> ASLTEIEHLVQSVCKSYRETCQLRLEDLLRQRSNIFSREEVTGYQRKSMWEMWERCAHHLTEAIQYVVEFAKRLSGFMELCQNDQIVLLKAGAMEVVLVRMCRAYNADNRTVFFEGKYGGMELFRALGCSELISSIFDFSHSLSALHFSEDEIALYTALVLINAHRPGLQEKRKVEQLQYNLELAFHHHLCKTHRQSILAKLPPKGKLRSLCSQHVERLQIFQHLHPIVVQAAF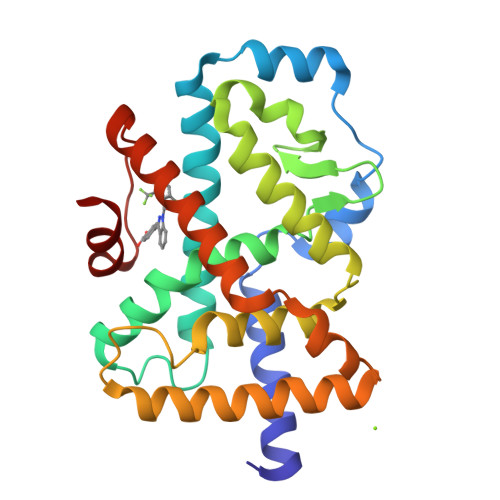PPLYKELFS> SNVRATYTVIFKNASGLPNGYDNWGWGCTLSYYGGAMIINPQEGKYGAVSLKRNSGSFRGGSLRFDMKNEGKVAILVENSEA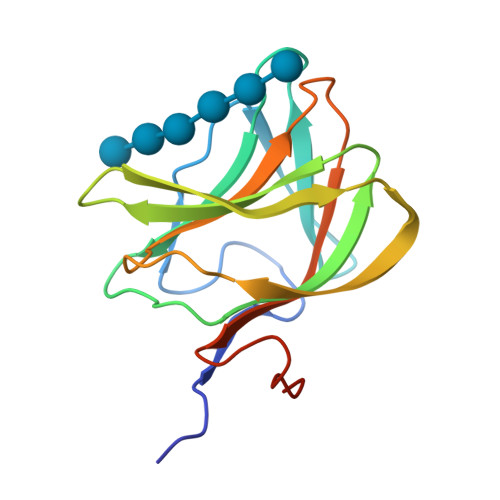DEKFEVETISPSDEYVTYILDVDFDLPFDRIDFQDAPGNGDRIWIKNLVHSTGSADDFVDPINLEHH>[4x]MTQGLLAGKRFLIAGVASKLSIAYGIAQALHREGAELAFTYPNEKLKKRVDEFAEQFGSKLVFP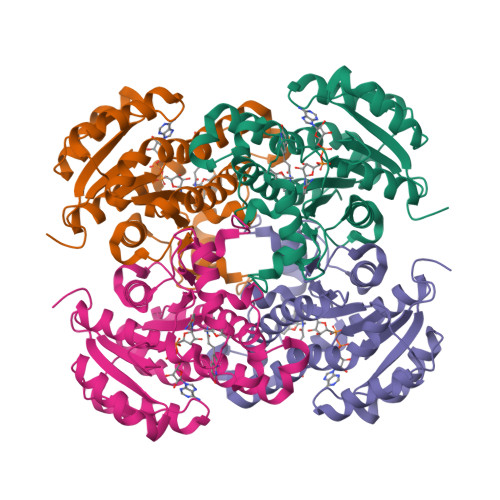CDVAVDAEIDNAFAELAKHWDGVDGVVHSIGFAPAHTLDGDFTDVTDRDGFKIAHDISAYSFVAMARAAKPLLQARQGCLLTLTYQGSERVMPNYNVMGMAKASLEAGVRYLASSLGVDGIRVNAISAGPIRTLAASGIKSFRKMLDANEKVAPLKRNVTIEEVGNAALFLCSPWASGITGEILYVDAGFNTVGMSQSMMDDE(2R)-2,4-dihydroxy-N-[(3S)-3-hydroxy-4-phenylbutyl]-3,3-dimethylbutanamide | C16 H25 N O4 | 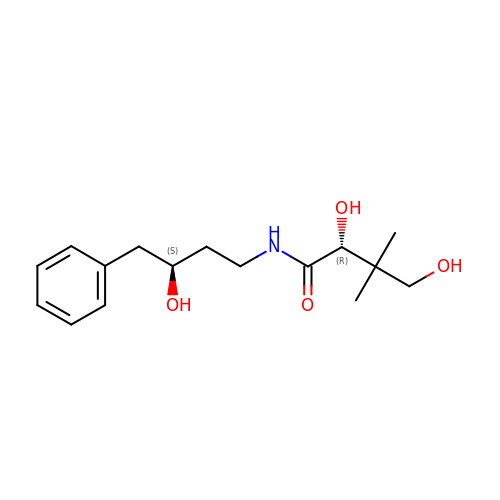VPOXPYKLLDGWBA-KGLIPLIRSA-N(E)-N-({3-hydroxy-2-methyl-5-[(phosphonooxy)methyl]pyridin-4-yl}methylidene)-L-alanine | C11 H15 N2 O7 P | 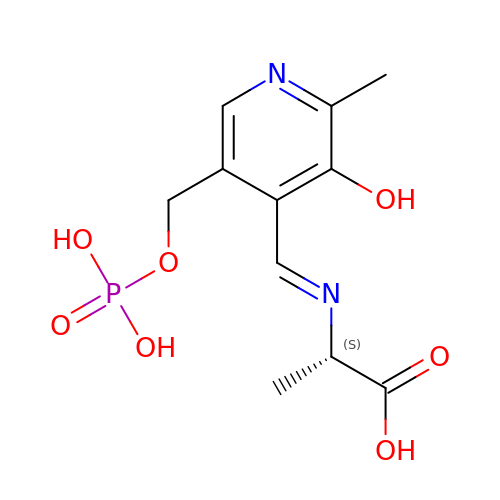UPOKXKNJCNHZTH-ASMSWWRESA-N ethyl (2Z,4S)-4-[(N-{[(2-cyclopropylethyl)amino](oxo)acetyl}-L-phenylalanyl)amino]-5-[(3S)-2-oxopyrrolidin-3-yl]pent-2-enoate 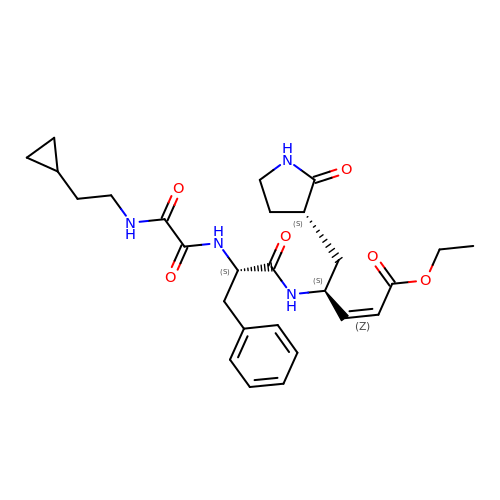| C27 H36 N4 O6 | HYAHTJFZAHAFHT-BDTNDASRSA-N>MFHTVDVKGVQTRYFDDGQDKDPILLIHGGHFGFFIPVGIESWGNVLEDFGEYGRVLAVDKLGQGETGLPLNDEDWTVDAVAEHVANFATQLGLKNLTLVGHSRGGMTAVLLALKYPEMVKKLVIISSATAAPAPPVGTDMDFYERVERTAPGGSAELIRHYHAAQAVNEGDLPEDYIGIATKWLESEKQLDAVAGYARNAEEHWLPSLSEGRRWVQERLADAGIPVPTLVVWGVNNRSAPVSMGKGLFDLIAANTLDSSLYLINNAGHHVFSDQREKFNAAVGAFISL[4x]

MehpH is a monoalkyl phthalate hydrolases discovered from Gordonia sp. Strain P8219, a Gram-positive bacteria, and able to dissimilate several different kinds of monoester, such as MBP, MEP and MEHP18. Here we report the structures of MehpH, a monoalkyl phthalate (MBP) hydrolase that catalyzes the reaction of MBP to phthalic acid and the corresponding alcohol, in apo and ligand-bound form. The structure of MehpH, determined at a resolution of 2.3 Å, exhibits the typical fold of the α/β hydrolase superfamily and is composed of an α/β hydrolase core (residues 24-152 and 225-311) and an α-helical lid domain (residues 153-224). The tunnel is narrow in the body of the structure, but significantly enlarged at the substrate entrance, due to the flexibility of the NC-loop. The catalytic triad, composed of Ser125, Asp259 and His291 with His291 bridging Asp259 and Ser125 through hydrogen bonds, is situated at the bottle-neck of the tunnel, suggesting this tunnel may be involved in the hydrolysis process of MehpH.

A catalytically inactive nucleophile mutation D259N was introduced in the active site to capture the transition state of MehpH-MBP interaction, and the subsequent structure was finally determined at a resolution of 2.8 Å. Structure superposition of the apo and ligand-bound MehpH revealed no significant conformational change on the whole structure of MehpH, except for the stabilization of the NC-loop in the lid domain and formation of a narrow hole extending from the protein surface to the catalytic Ser125. Surprisingly, instead of a separate electron density for MBP in the catalytic center, we observed extra electron density on the side chain of Ser125, indicative of an intermediate trapped in the structure. The shape of the electron density is consistent with that of PA, suggesting that Ser125 is covalent modified by PA. Additionally, adjacent to the catalytic center, we discovered the electron density of butanol in the penetrating tunnel. It appears that the butanol is highly dynamic in the structure, as only one butanol molecule with intact electron density in the four MehpH of a single asymmetric unit. PA is tightly embedded in a positively charged pocket that is made up of residues His53, Phe56, Ser125, Arg126, Thr152 and His291 from the α/β hydrolase core and Asp162, Met163 and Tyr166 from the lid domain. Particularly, Arg126 and Asp162 construct a gate to lock PA in the pocket through two hydrogen bonds formed by their side chains. In contrast to the extensive interactions of PA with MehpH, the butanol is only engaged one hydrogen bond with Tyr166. Of note, the location of the butanol is very close to His291 of the triad, leaving no space for a water molecule to attach the Ser125-PA intermediate.>[4x]SPNPLDVSKTYPTLHILLQFNHRGLEARIFRHGQLWAETHAEVVLRSKTKQISFLSNGSYPSMDATTPLNPWKSTYQAVLRAEPHRVTMDVYHKRIRPFRLPLVQKEWRTCEENVFGLYHVFETHYAGYFSDLLIHDVETNPGGSKHHHHHH

Programmed –1 ribosomal frameshifting (PRF) in cardioviruses is activated by the 2A protein, a multi-functional virulence factor that also inhibits cap-dependent translational initiation. Cardioviruses present a highly unusual variation to conventional viral PRF in which the virally encoded 2A protein is required as an essential trans-activator. The PRF-stimulatory activity of 2A is related to its ability to bind to the RNA stimulatory element. Here we show that 2A adopts an RNA-binding fold, allowing specific recognition and stabilisation of the PRF stimulatory element in the viral RNA and direct binding to host ribosomes.

Here we present the crystal structure of 2A from encephalomyocarditis virus (EMCV), revealing a novel RNA-binding fold that we term a “beta-shell”. We crystallised the protein and determined the structure by multiple-wavelength anomalous dispersion (MAD) analysis of a selenomethionyl derivative. The asymmetric unit (ASU) of the P6222 cell contains four copies of 2A related by non-crystallographic symmetry (NCS), and the structure was refined to 2.6 Å resolution. Unexpectedly, the four molecules are arranged as a pair of covalent ‘dimers’ with an intermolecular disulfide bond forming between surface-exposed cysteine residues (C111). This arrangement is likely an artefact of crystallisation, which took >30 days, possibly due to the gradual oxidation of C111 promoting formation of the crystalline lattice. 2A adopts a compact, globular fold of the form β3αβ3αβ. The most striking feature is a curved, seven-stranded anti-parallel beta sheet. The concave face of the beta sheet is supported by tight packing against the two alpha helices: together, this comprises the hydrophobic core of the fold. In contrast, the solvent-exposed convex face and surrounding loops are enriched with arginine, lysine and histidine residues, conferring a strong positive electrostatic surface potential at physiological pH. In addition to the N- and C- termini, the β2-loop-β3 region (residues 28–37) exists in multiple conformations that deviate by up to 5.8 Å in the position of the Cα backbone.>[4x]MIFTKEPANVFYVLVSAFRSNLCDEVNMSRHRHMVSTLRAAPGLYGSVESTDLTGCYREAI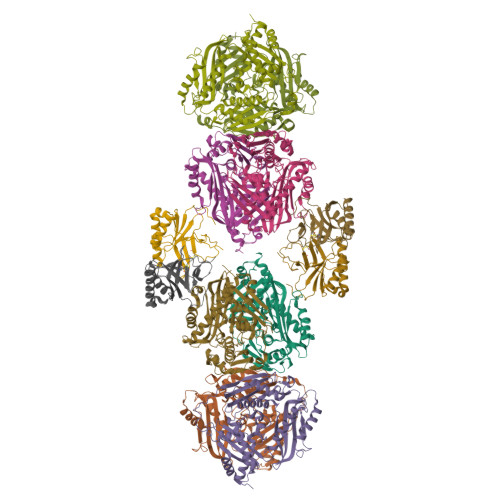SSAPTEEKTVRVRCKDKAQALNVARLACNEWEQDCVLVYKSQTHTAGLVYAKGIDGYKAERLPGSFQEVPKGAPLQGCFTIDEFGRRWQVQHHHHHH;>MAKHLFTSESVSEGHPDKIADQISDAVLDAILEQDPKARVACETYVKTGMVLVGGEITTSAWVDIEEITRNTVREIGYVHSDMGFDANSCAVLSAIGKQSPDINQGVDRADPLEQGAGDQGLMFGYATNETDVLMPAPITYAHRLVQRQAEVRKNGTLPWLRPDAKSQVTFQYDDGKIVGIDAVVLSTQHSEEIDQKSLQEAVMEEIIKPILPAEWLTSATKFFINPTGRFVIGGPMGDCGLTGRKIIVDTYGGMARHGGGAFSGKDPSKVDRSAAYAARYVAKNIVAAGLADRCEIQVSYAIGVAEPTSIMVETFGTEKVPSEQLTLLVREFFDLRPYGLIQMLDLLHPIYKETAAYGHFGREHFPWEKTDKAQLLRDAAGLKHHHHHH[8x]> X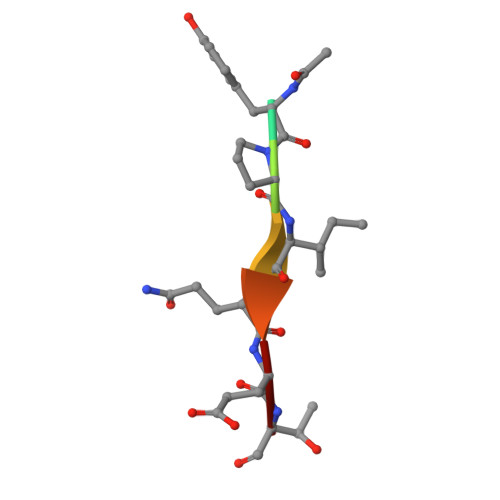YPIQET>SNAMKEKVVSLAQDLIRRPSISPNDEGCQQIIAERLEKLGFQIEWMPFNDTLNLWAKHGTSEPVIAFAGH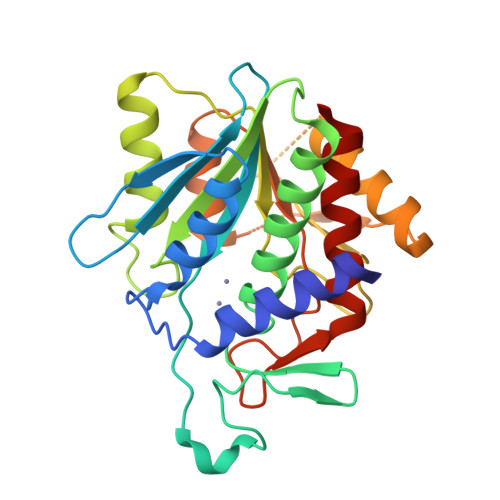TDVVPTGDENQWSSPPFSAEIIDGMLYGRGAADMKGSLAAMIVAAEEYVKANPNHKGTIALLITSDEEATAKDGTIHVVETLMARDEKITYCMVGEPSSAKNLGDVVKNGRRGGGFLTKPGKLLDSITSAIEETIGITPKAETGGGTSDGRFIALMGAEVVEFGPLNSTIHKVNECVSVEDLGKCGEIYHKMLVNLLDS[2x]methyl 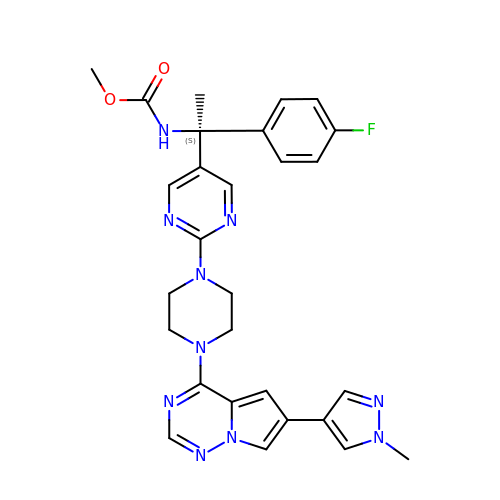~{N}-[(1~{S})-1-(4-fluorophenyl)-1-[2-[4-[6-(1-methylpyrazol-4-yl)pyrrolo[2,1-f][1,2,4]triazin-4-yl]piperazin-1-yl]pyrimidin-5-yl]ethyl]carbamate | C28 H29 F N10 O2 | KTPLYBJJFYLCFB-NDEPHWFRSA-N> MMLQHTSLLCRKALQSYPVPPRARNYERRWSSS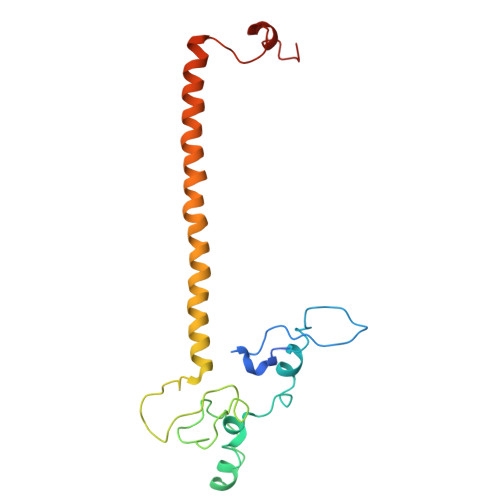RTNPYNRMFWRTVLNEDFARPSFWVSDFRHKYLAKHGMDYQGRVPASPAPGMYQGFSDVHKILANHPKPQRESRHLPVMPMTPRVVFEHAQEKRIDYAKKMHRDRRLVEQLRTHEFWGWYMKLQRVRGRWCKEHGVSSRGVYGPAVDAAELWG>MVIKFGYKASAEQFGPRELVELGVLAEAHGMDSATVSDHFQPWRHEGGHAPFSLAWMTAVGERTSRLQLGTSVMTPTFRYNPAVVAQAFATMGCLYPGRIMLGVGTGEALNEIATGFAGEWPEFKERFARLREAVALMRELWLGDRVDFEGNYYKTVGASIYDVPEGGIPVYIAAGGPVVARYAGRSGDGFICTSGKGMELYTEKLMPAVAEGAEKADRDVAEIDKMIEIKISYDTDPELALENTRFWAPLSLTPEQKHSIDDPIEMERAADALPIEQVAKRWIVASDPDE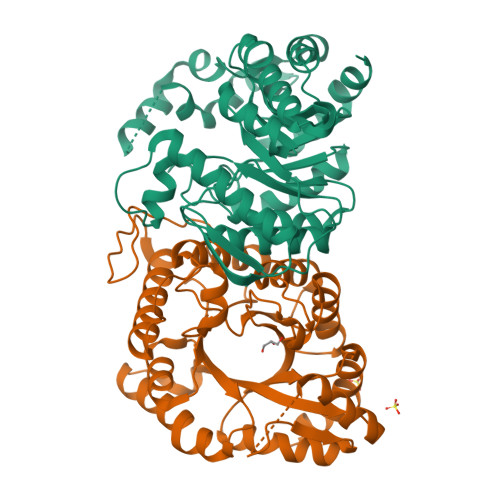AVAQIRPYLDAGLNHLVFHAPGHDQKRFLELFQRDLAPRLRGLA[2x]Using X-ray crystallography, we show that the ciliopathy-associated centriolar protein CEP120 contains three C2 domains. CEP120, for example, plays a key role in the duplication, elongation, and maturation of centrioles, which in principle could impact the production of a functional basal body (Comartin et al., 2013, Lin et al., 2013, Mahjoub et al., 2010, Wu et al., 2014). All three C2 domains of CEP120 (C2A, C2B, and C2C) adopt the PLC δ1-like topology II and are structurally similar to each other (root-mean-square deviation [RMSD], 2.4–2.6 Å), with major differences found mainly in their loop length. Thus, the CEP120 C2 domains probably play a role as protein-protein interaction modules.

For the O.n.-A200P mutant (equivalent to the H.s.-A199P JATD mutation), we obtained diffraction-quality crystals that allowed a successful structure determination to a resolution of 2.1 Å. To obtain this crystal form, we introduced an additional mutation (G307S) that we found serendipitously. Residue G307 is solvent exposed and is not strictly conserved. Furthermore, the crystal structure of O.n. CEP120 C2B G307S did not reveal significant structural differences when compared to the corresponding wild-type (WT) structure (RMSD, 0.19 Å with 181 aligned residue pairs).

> GPHMPEKLEAILIPDQGYHQVGPADLCTDMFVLSVTVAFATKLEQLVPSTMKLSAEGSEFFFYYSLLGNDITSEPFHNLLSPDFEPERASVRIRSSKQILKAFLSQQPSLQIHLCCGNHSLGSTDVSLSALAGISTDLDNKAATVESAFILQPPKRVKQTLPALPTDLQPTLGVAVTLRREEVALQQSVGNKE ethyl (5R)-5-(4-cyanophenyl)-7-methyl-8-[3-(trifluoromethyl)phenyl]-1,5-dihydroimidazo[1,2-a]pyrimidin-4-ium-6-carboxylate | C24 H20 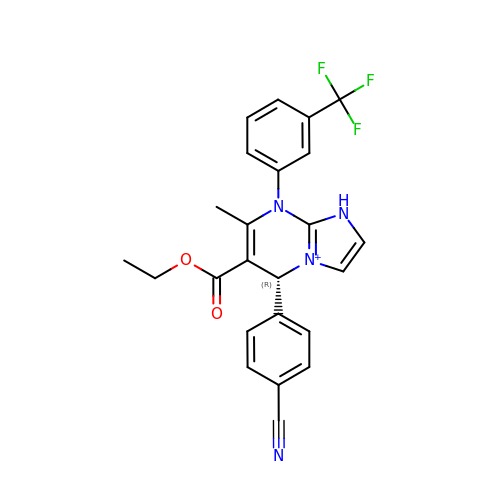F3 N4 O2 | JHIVXCHUXFMPOR-OAQYLSRUSA-O S-[(2E,6E,10E)-14-(dimethylamino)-3,7,11-trimethyltetradeca-2,6,10-trien-1-yl] 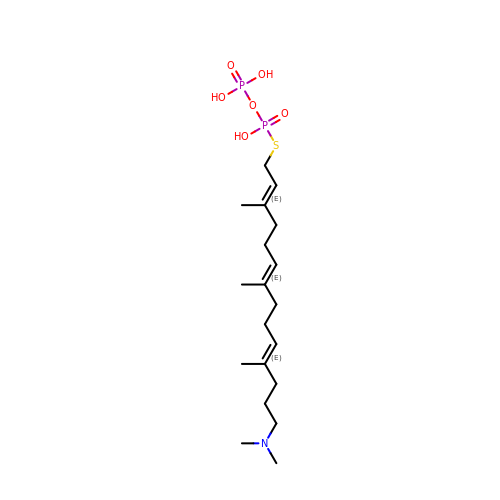trihydrogen thiodiphosphate | C19 H37 N O6 P2 S | WNRLOKILDUQQLN-WNWLUAIZSA-N>[23x]MASWSHPQFEKIEGRMSVTVPN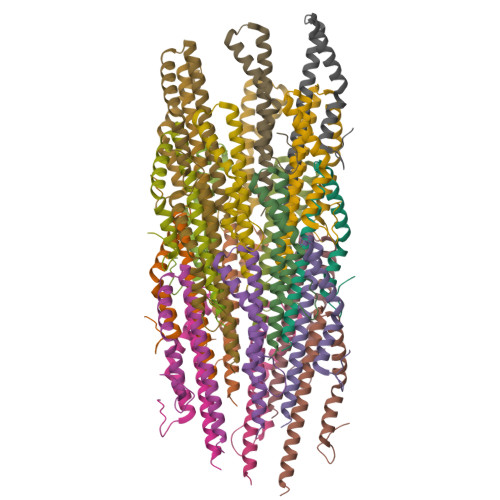DDWTLSSLSETFDDGTQTLQGELTLALDKLAKNPSNPQLLAEYQSKLSEYTLYRNAQSNTVKVIKDVDAAIIQNFR>[4x]MTSATASFATRTSLAADLAALGLAWGDAIMVHAAVSRVGRLLDGPDTIIAALRDTVGPGGTVLAYADWEARYEDLVDDAGRVPPEWREHVPPFDPQRSRAIRDNGVLPEFLRTTPGTLRSGNPGASLVALGAKAEWFTADHPLDYG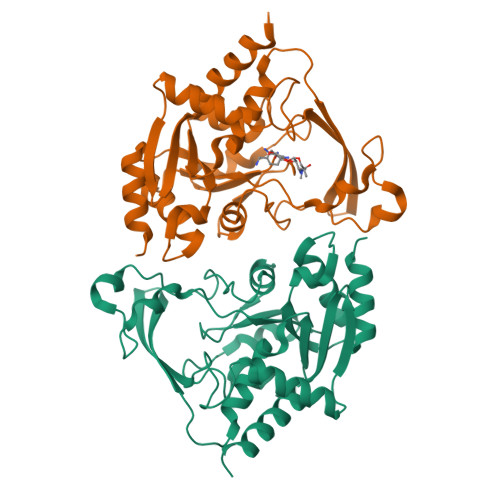YGEGSPLAKLVEAGGKVLMLGAPLDTLTLLHHAEHLADIPGKRIKRIEVPFATPTGTQWRMIEEFDTGDPIVAGLAEDYFAGIVTEFLASGQGRQGLIGAAPSVLVDAAAITAFGVTWLEKRFGTPSP(2R,3R,4S)-2-({[(1S)-2-HYDROXY-1-PHENYLETHYL]AMINO}METHYL)PYRROLIDINE-3,4-DIOL 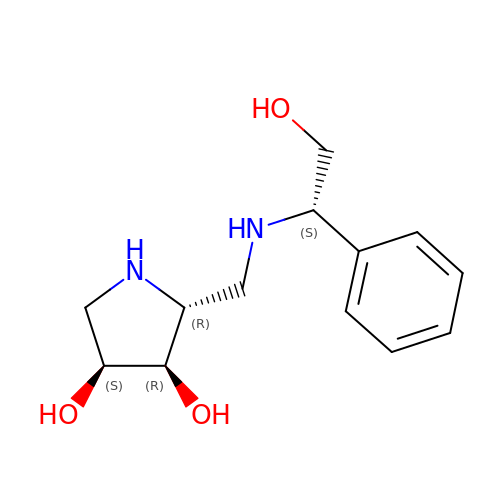| C13 H20 N2 O3 | OGMKEJTXCCFISS-FVCCEPFGSA-N(5S)-5-(difluoromethoxy)pyridin-2(5H)-one | C6 H5 F2 N O2 | 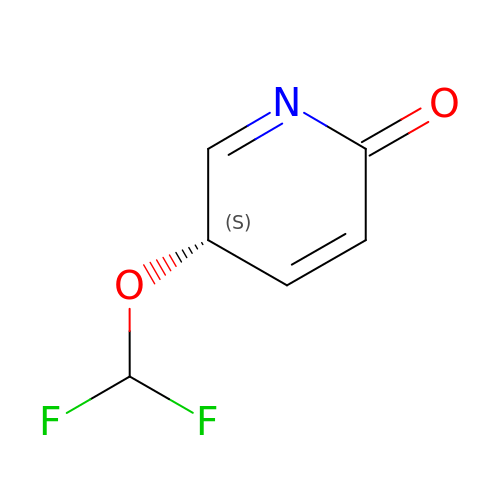LTVXNUWMTTYHRL-BYPYZUCNSA-N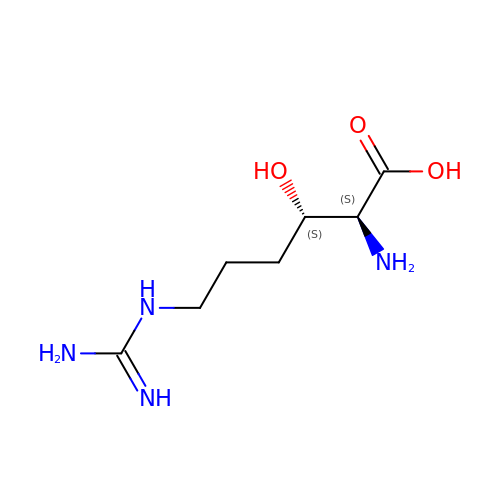(3S)-N~6~-carbamimidoyl-3-hydroxy-L-lysine | C7 H16 N4 O3 | ZMNNJGSTNCXCMN-WHFBIAKZSA-N>[2x]MMEQVCDVFDIYAICACCKVESKNEGKKNEVFNNYTFRGLGNKGVLPWKCISLDMKYFRAVTTYVNESKYEKLKYKRCKYLNKETVDNVNDMPNSKKLQNVVVMGRTNWESIPKKFKPLSNRINVILSRTLKKEDFDEDVYIINKVEDLIVLLGKLNYYKCFILGGSVVYQEFLEKKLIKKIYFTRINSTYECDVFFPEINENEYQIISVSDVYTSNNTTLDFIIYKKTNNKMLNEQNCIKGEEKNNDMPLKNDDKDT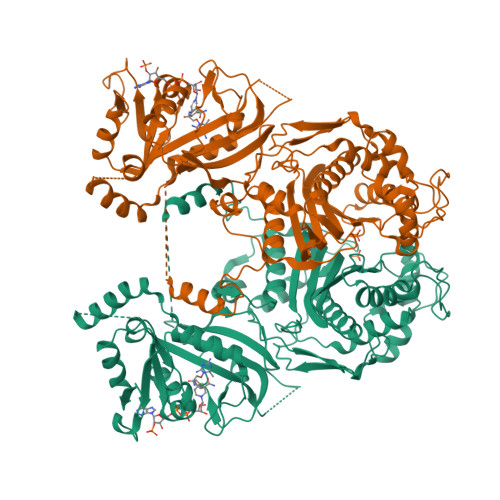CHMKKLTEFYKNVDKYKINYENDDDDEEEDDFVYFNFNKEKEEKNKNSIHPNDFQIYNSLKYKYHPEYQYLNIIYDIMMNGNKQSDRTGVGVLSKFGYIMKFDLSQYFPLLTTKKLFLRGIIEELLWFIRGETNGNTLLNKNVRIWEANGTREFLDNRKLFHREVNDLGPIYGFQWRHFGAEYTNMYDNYENKGVDQLKNIINLIKNDPTSRRILLCAWNVKDLDQMALPPCHILCQFYVFDGKLSCIMYQRSCDLGLGVPFNIASYSIFTHMIAQVCNLQPAQFIHVLGNAHVYNNHIDSLKIQLNRIPYPFPTLKLNPDIKNIEDFTISDFTIQNYVHHEKISMDMAA>GAMAVYPCGICTNEVNDDQDAILCEASCQKWFHRICTGMTETAYGLLTAEASAVWGCDTCMAD[2x];>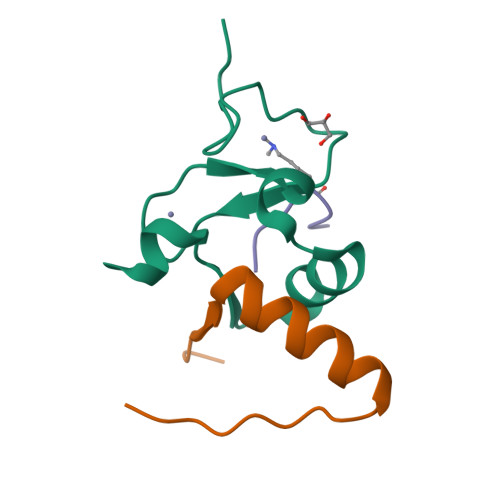GAMVYVFSTEMANKAAEAVLKGQVETIVSFHI[2x];>[2x]ARTKQTA>ISLNQQRMNGVVAALKQSNARRVIDLGCGQGNLLKILLKDSFFEQITGVDVSYRSLEIAQERLDRLRLPRNQWERLQLIQGALTYQDKRFHGYDAATVIEVIEHLDLSRLGAFERVLFEFAQPKIVIVTTPNIEYNVKFANLPA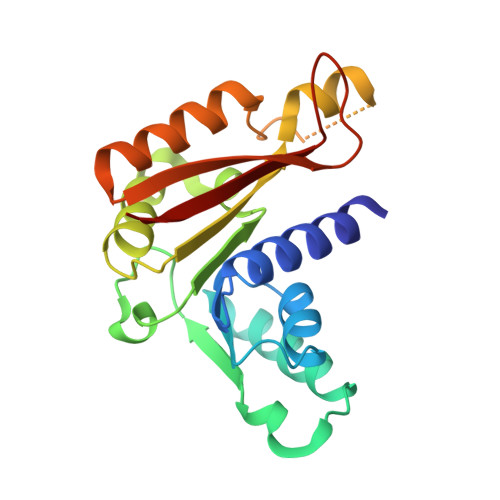GKLRHKDHRFEWTRSQFQNWANKITERFAYNVQFQPIGEADPEVGSPTQMAVFIHRGH[2x]2,6-dimethylphenol | C8 H10 O | 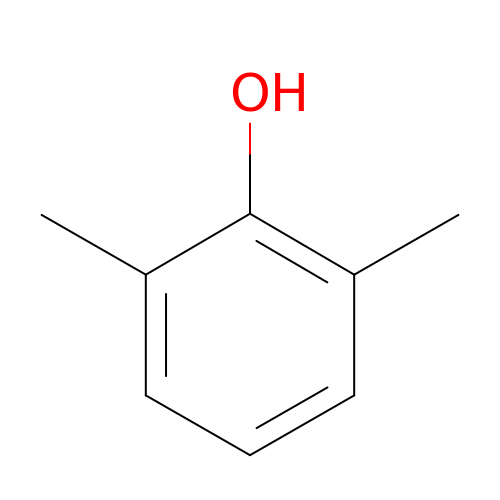NXXYKOUNUYWIHA-UHFFFAOYSA-N>MPDFLGHAENPLREEEWARLNETVIQVARRSLVGRRILDIYGPLGAGVQTVPYDEFQGVSPGAVDIVGEQETAMVFTDARKFKTIPIIYKDFLLHWRDIEAARTHNMPLDVSAAAGAAALCAQQEDELIFYGDARLGYEGLMTANGRLTVPLGDWTSPGGGFQAIVEATRKLNEQGHFGPYAVVLSPRLYSQLHRIYEHHHVLEIETIRQLASDGVYQSNRLRGESGVVVSTGRENMDLAVSMDM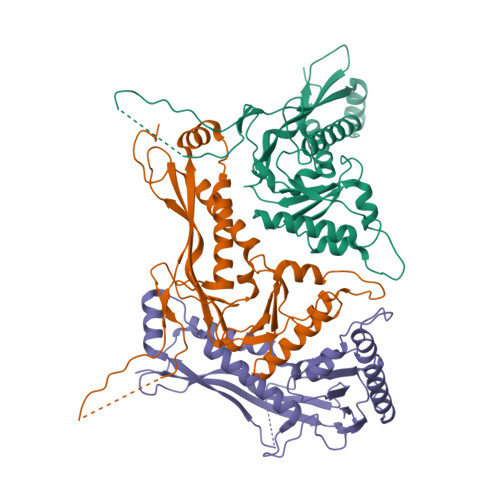VAAYLGASRMNHPFRVLEALLLRIKHPDAICTLEGAGATERR[3x]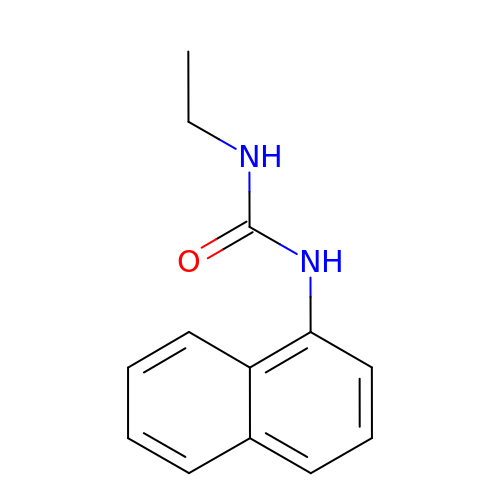1-ethyl-3-naphthalen-1-ylurea | C13 H14 N2 O | SMNYGFHWZXVHCR-UHFFFAOYSA-N> GEIQWMRPSKEVGYPIINAPSKTKLEPSAFHYVFEGVKEPAVLTKNDPRLKTDFEEAIFSKYVGNKITEVDEYMKEAVDHYAGQLMSLDINTEQMCLEDAMYGTDGLEALDLSTSAGYPYVAMGKKKRDILNKQTRDTKEMQKLLDTYGINLPLVTYVKDELRSKTKVEQGKSRLIEASSLNDSVAMRMAFGNLYAAFHKNPG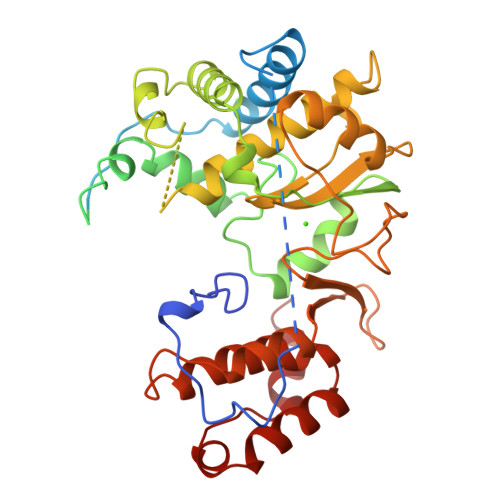VITGSAVGCDPDLFWSKIPVLMEEKLFAFDYTGYDASLSPAWFEALKMVLEKIGFGDRVDYIDYLNHSHHLYKNKTYCVKGGMPSGCSGTSIFNSMINNLIIRTLLLKTYKGIDLDHLKMIAYGDDVIASYPHEVDASLLAQSGKDYGLTMTPADKSATFETVTWENVTFLKRFFRADEKYPFLIHPVMPMKEIHESIRWTKDPRNTQDHVRSLCLLAWHNGEEEYNKFLAKIRSVPIGRALLLPEYSTLYRRWLDSF>MVMTTAGYYAAVDWGTSSFRLWIIGEDGAVLAERRSAEGMTTAAKTGFHTILDGHLAAVSAPAHLPIIICGMAGARQGWKEAGYIETPAALAEIAGRATAIPDVDRDIRILPGLAQRDRRHPDVMRGEETQLLGAAAHLGAGSHLVCMPGTHSKWVRLADDRVEGFSTFMTGELFDTIARHTILSHAVAEADTFAAGSAAFTDAVSRTRENPALATNLLFSVRAGQLLHGTAAADARAQLSGTLIGLEIAGALAGSGSVDGVCLVGSGGLGTLYRTALESQGLNVRAVDAD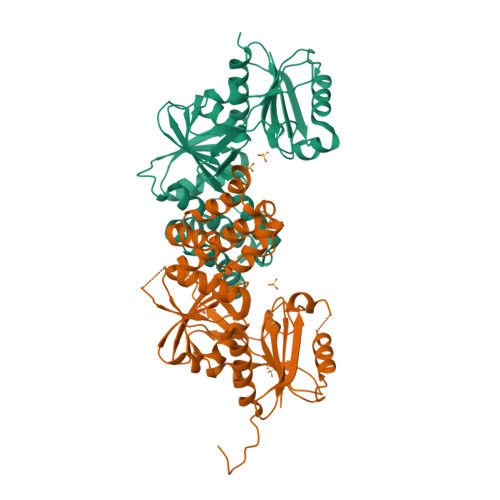EAVRAGLSAAARAIWPLAENLYFQSHHHHHHWSHPQFEK[2x]{[-(BIS-CARBOXYMETHYL-AMINO)-ETHYL]-CARBOXYMETHYL-AMINO}-ACETIC ACID | C10 H16 N2 O8 | 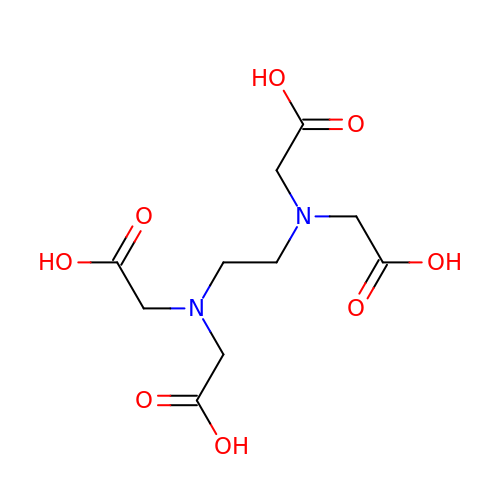KCXVZYZYPLLWCC-UHFFFAOYSA-N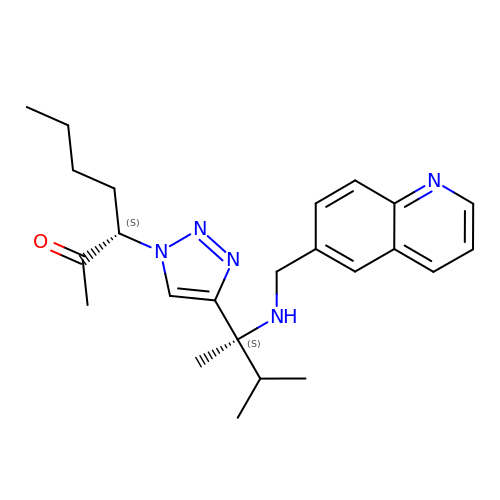(3S)-3-(4-{(1S)-1,2-dimethyl-1-[(quinolin-6-ylmethyl)amino]propyl}-1H-1,2,3-triazol-1-yl)heptan-2-one | C24 H33 N5 O | XHOTUPQHXLRCJV-UPVQGACJSA-N>DYKDDDDKLHSQANLMRLKSDLFNRSPMYPGPTKDDPLTVTLGFTLQDIVKADSSTNEVDLVYYEQQRWKLNSLMWDPNEYGNITDFRTSAADIWTPDITAY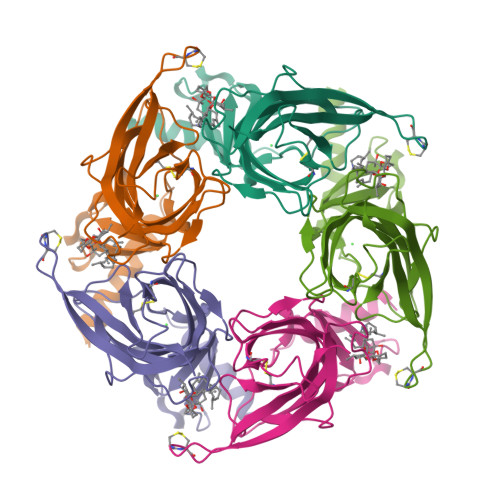SSTRPVQVLSPQIAVVTHDGSVMFIPAQRLSFMCDPTGVDSEEGATCAVKFGSWVYSGFEIDLKTDTDQVDLSSYYASSKYEILSATQTRQVQHYSCCPEPYIDVNLVVKFRERRAGNGFFRNLFD[10x]> MKDLLKFLKAQTKTEEFDAIKIALASPDMIRSWSFGEVKKPETINYRTFKPERDGLFCARIFGPVKDYECLCGKYKRLKHRGVICEKCGVEVTQTKVRRERMGHIELASPTAHIWFLKSLPSRIGLLLDMPLRDIERVLYFESYVVIEGGMTNLERQQILTEEQYLDALEEFGDEFDAKMGAEAIQALLKSMDLEQECEQLREELNETNSETKRKKLTKRIKLLEAFVQSGNKPEWMILTVLPVLPPDLRPLVPLDGGRFATSDLNDLYRRVINRNNRLKRLLDLAAPDIIVRNEKRMLQEAVDALLDNGRRGRAITGSNKRPLKSLADMIKGKQGRFRQNLLGKRVDYSGRSVITVGPYLRLHQCGLPKKMALELFKPFIYGKLELRGLATTIKAAKKMVEREEAVVWDILDEVIREHPVLLNRAPTLHRLGIQAFEPVLIEGKAIQLHPLVCAAYNADFDGDQMAVHVPLTLEAQLEARALMMSTNNILSPANGEPIIVPSQDVVLGLYYMTRDCVNAKGEGMVLTGPKEAERLYRSGLASLHARVKVRITEYEKDANGELVAKTSLKDTTVGRAILWMIVPKGLPYSIVNQALGKKAISKMLNTCYRILGLKPTVIFADQIMYTGFAYAARSGASVGIDDMVIPEKKHEIISEAEAEVAEIQEQFQSGLVTAGERYNKVIDIWAAANDRVSKAMMDNLQTET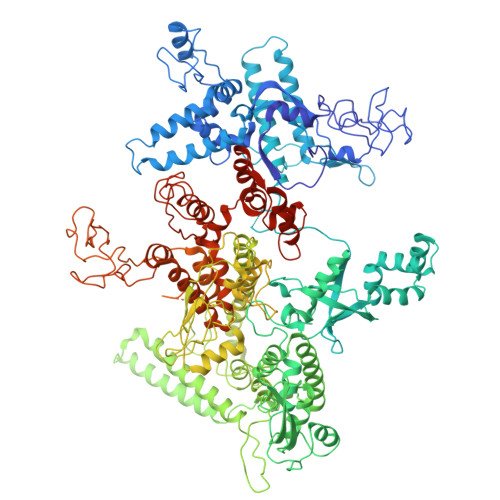VINRDGQEEKQVSFNSIYMMADSGARGSAAQIRQLAGMRGLMAKPDGSIIETPITANFREGLNVLQYFISTHGARKGLADTALKTANSGYLTRRLVDVAQDLVVTEDDCGTHEGIMMTPVIEGGDVKEPLRDRVLGRVTAEDVLKPGTADILVPRNTLLHEQWCDLLEENSVDAVKVRSVVSCDTDFGVCAHCYGRDLARGHIINKGEAIGVIAAQSIGEPGTQLTMRTFHIGGAASRAAAESSIQVKNKGSIKLSNVKSVVNSSGKLVITSRNTELKLIDEFGRTKESYKVPYGAVLAKGDGEQVAGGETVANWDPHTMPVITEVSGFVRFTDMIDGQTITRQTDELTGLSSLVVLDSAERTAGGKDLRPALKIVDAQGNDVLIPGTDMPAQYFLPGKAIVQLEDGVQISSGDTLARIPQESGGTKDITGGLPRVADLFEARRPKEPAILAEISGIVSFGKETKGKRRLVITPVDGSDPYEEMIPKWRQLNVFEGERVERGDVISDGPEAPHDILRLRGVHAVTRYIVNEVQDVYRLQGVKINDKHIEVIVRQMLRKATIVNAGSSDFLEGEQVEYSRVKIANRELEANGKVGATYSRDLLGITKASLATESFISAASFQETTRVLTEAAVAGKRDELRGLKENVIVGRLIPAGTGYAYHQDRMRRRAAGEAPAAPQVTAEDASASLAELLNAGLGGSDNE>[2x]GSKEGEYIKLKVIGQDSSEIHFKVKMTTHLKKLKES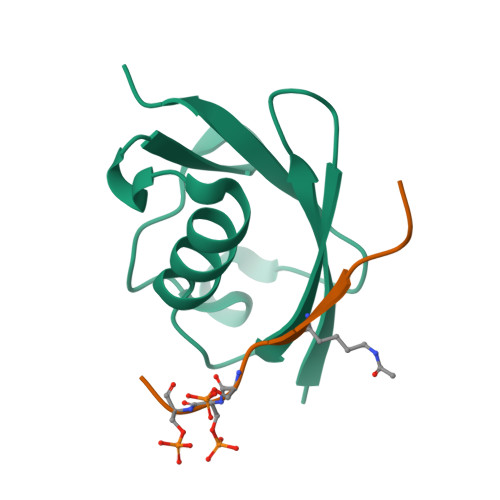YAQRQGVPMNSLRFLFEGQRIADNHTPKELGMEEEDVIEVYQEQTGG;>GSGAGEAEERVVVISSSEDSDAENSSSRY[2x]>[4x]GVADASDPIRPLVEALNAEAPLKLWSVLVTCLGDVS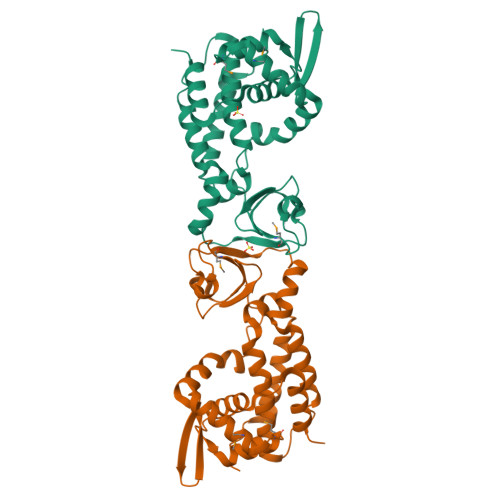RDGVIEVSGVALSSFVERMGLQPQAMRVALHRLKRDGWVESRRLGRVGFHRLSDSALTQTRAVAGRIYGPGAGPAPWHLAGMPPDAPDGLSLLPDTLSATPISRRFALICGPLEDVPEDWLLTAPSGRGLPVWVQDVVVEAGCEAEFKALERTLAQIDKVPDTRLERFTLRVLVLHAWRRLILRSSPAAEAALGGARAEISCRARVHQLLDQLGSVEPDWDLPATEDAAS>[2x]MEALVLVGHGSRLPYSKELLVKLAEKVKERNLFPIVEIGLMEFSEPTIPQAVKKAIEQGAKRIIVVPVFLAHGIHTTRDIPRL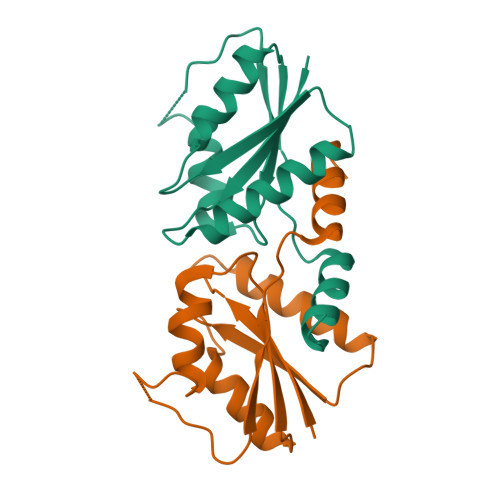LGLIEDNHEHHHEHSHHHHHHHHHEHEKLEIPEDVEIIYREPIGADDRIVDIIIDRAFGR methyl {3-[2-(acetylamino)ethyl]-2-iodo-1H-indol-5-yl}carbamate | C14 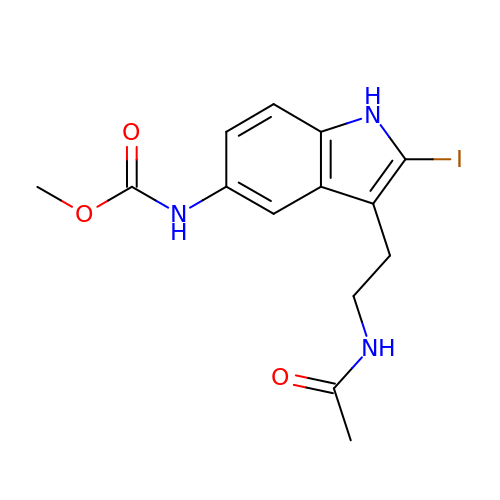H16 I N3 O3 | BMRSKORHUNWKLU-UHFFFAOYSA-N>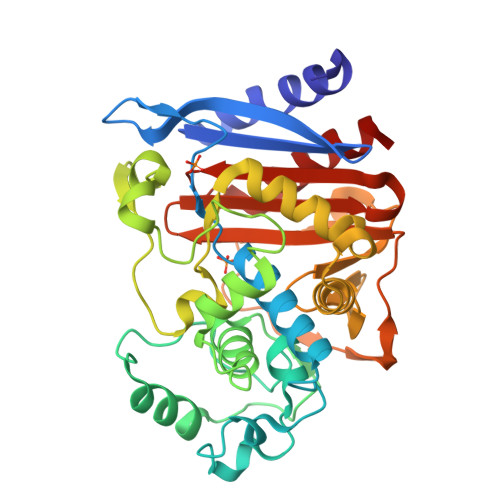[2x]APQQINDIVHRTITPLIEQQKIPGMAVAVIYQGKPYYFTWGYADIAKKQPVTQQTLFELGSVSRTFTGVLGGDAIARGEIKLSDPTTKYWPELTAKQWNGITLLHLATYTAGGLPLQVPDEVKSSSDLLRFYQNWQPAWAPGTQRLYANSSIGLFGALAVKPSGLSFEQAMQTRVFQPLKLNHTWINVPPAEEKNYAWGYREGKAVHVSPGALDAEAYGVKSTIEDMARWVQSNLKPLDINEKTLQQGIQLAQSRYWQTGDMYQGLGWEMLDWPVNPDSIINGSDNKIALAARPVKAITPPTPAVRASWVHKTGATGGFGSYVAFIPEKELGIVMLANKNYPNPARVDAAWQILNALQ>GMDQESNATSQDILKQHAAHYESDMGGLPEALVQLAEYAPETFDAYSRMRTTMLKSEADGAKLPLKYKHLILVVLDAIRDEPIGIVNHTRAAMNAGLSVDELIEGILLGIIVYGMPAWG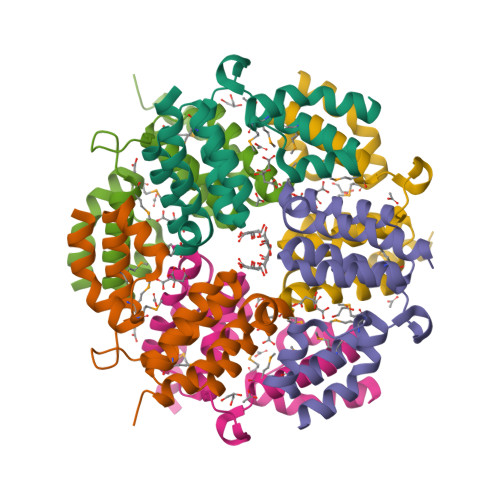KTGRKAVTFAVEFEKELAGKRT[3x]> GSQIPASEQETLVRPKPLLLKLLKSVGAQKDTYTMKEVLFYLGQYIMTKRLYDEKQQHIVYCSNDLLGDLFGVPSFSVKEHRK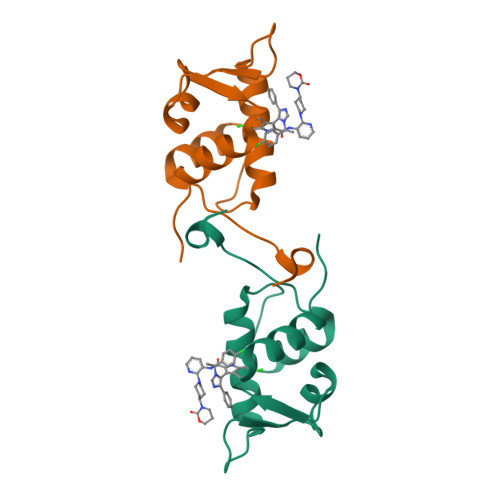IYTMIYRNLVVVN>[2x]VSSRVSTRSSLAEDLRAIGLADGDAVLVHAALRKVGKIVGGPDDILDAMRDVIGPAGTVLGYADWQLEDEIRDDPAMREHIPAFDPLRSRSIRDNGFWPELIRTTPGALRSASPGASMAAIGGEAEWFTADHALDYGYGPRSPL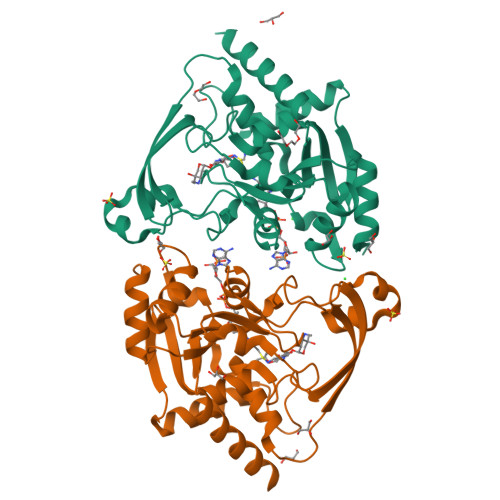GKLVEAKGKVLMLGAPLDTMTLLAHAEHLADFPNKRILRYEAPILVDGEKVWRWFEEFDTSDPPDGLADDYFAGIVEEFLATGRGKRGKIGEASSVLVPADEIVAFAVDWLERWGRTAR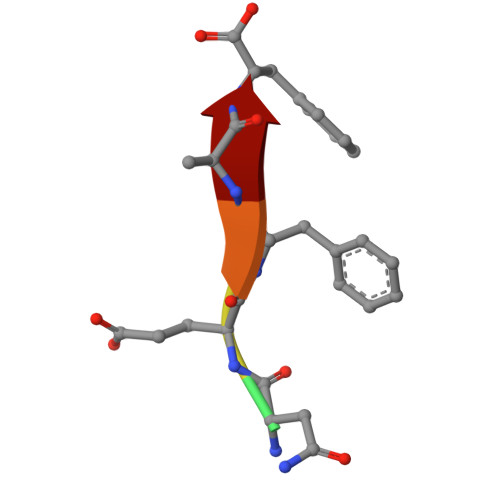> TNEFAF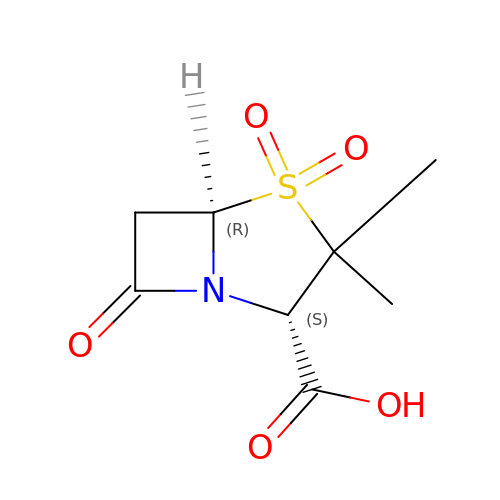SULBACTAM | C8 H11 N O5 S | FKENQMMABCRJMK-RITPCOANSA-N>[2x]GSKVEDPKDFPSELLSFLSHAVFSNRTLACFAIYTTKEKAALLYKKIMEKYSVTFISRHNSYNHNILFFLTP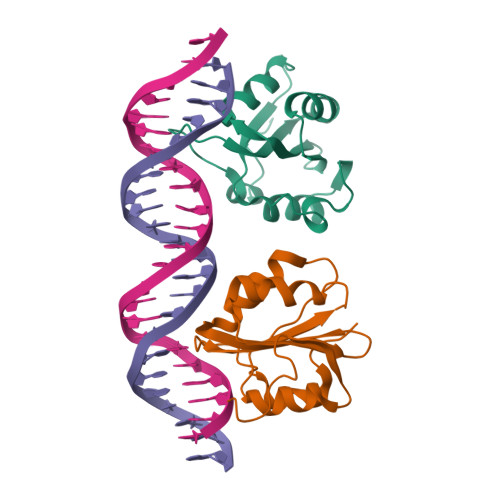HRHRVSAINNYAQKLCTFSFLICKGVNKEYLMYSALTRDPFSVIEESLPGGLKEHDFNPE>GSHPFNSEPPLTKLYDSGFLTPVSLHFVRNHGPVPYVPDENILDWEVSIEGMVETPYKIKLSDIMEQFDIYSTPVTMVCAGNRRKEQNMVKKGAGFNWGAAGTSTSLWTGCMLGDVIGKARPSKRARFVWMEGADNPANGAYGTCIRLSWCMDPERCIMIAYQQNGEWLHPDHGKPLRVVIPGVIGGRSVKWLKKLVVSDRPSENWYHYFDNRVLPTMVTPEMAKSDDRWWKDERYAIYDLNLQTIICKPENQQVIKI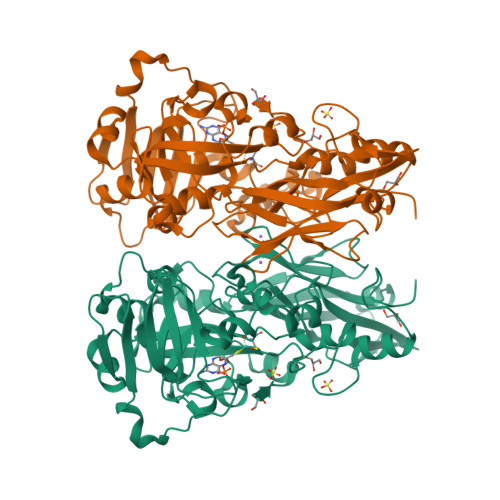SEDEYEIAGFGYNGGGVRIGRIEVSLDKGKSWKLADIDYPEDRYREAGYFRLFGGLVNVCDRMSCLCWCFWKLKVPLSELARSKDILIRGMDERMMVQPRTMYWNVTSMLNNWWYRVAIIREGESLRFEHPVVANKPGGWMDRVKAEGGDILDNNWGEVDDTGQAG[2x]>GSKGNVDLVFLFDGSMSLQPDEFQKILDFMKDVMKKLSNTSYQFAAVQFSTSYKTEFDFSDYVKWKDPDALLKHVKHML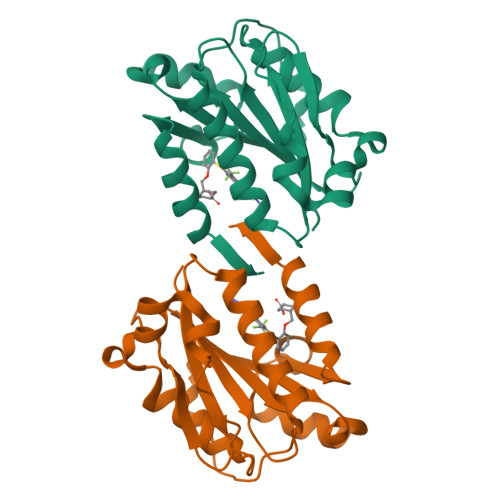LLTNTFGAINYVATEVFREELGARPDATKVLIIITDGEATDSGNIDAAKDIIRYIIGIGKHFQTKESQETLHKFASKPASEFVKILDTFEKLKDLFTELQKKIYVI[2x]>[6x]GSHMMIYPDEAMLYAPVEWHDCSEGFEDIRYEKSTDGIAKITINRPQVRNAFRPLTVKEMIQALADARYDDNIGVIILTGAGDKAFCSGGDQKVRGDYGGYKDDSGVHHLNVLDFQRQIRTCPKPVVAMVAGYSIGGGHVLHMMCDLTIAADNAIFGQTGPKVGSFDGGWGASYMARIVGQKKAREIWFLCRQYDAKQALDMGLV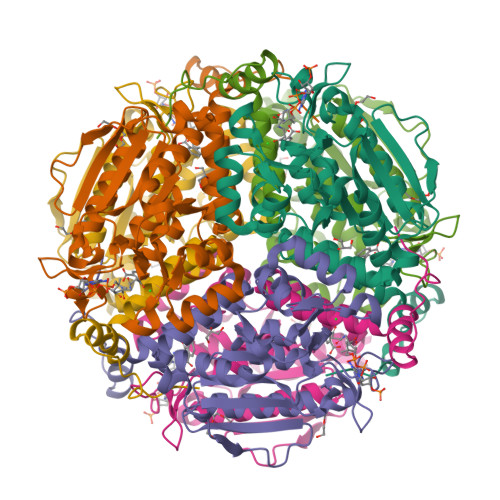NTVVPLADLEKETVRWCREMLQNSPMALRCLKAALNADCDGQAGLQELAGNATMLFYMTEEGQEGRNAFNQKRQPDFSKFKRNP The human AAA-ATPase Bcs1L translocates the fully assembled Rieske iron-sulfur protein (ISP) precursor across the mitochondrial inner membrane, enabling respiratory Complex III assembly. Bcs1L is a membrane-bound oligomer, with each subunit consisting of an N-terminal TM segment, a middle Bcs1-specific domain, and a C-terminal AAA domain that is highly distinct, forming a clade of its own in the broad AAA protein family. Here, we captured Bcs1L conformations by cryo-EM during active ATP hydrolysis in the presence or absence of ISP substrate. In contrast to the threading mechanism widely employed by AAA proteins in substrate translocation, subunits of Bcs1L alternate uniformly between ATP and ADP conformations without detectable intermediates that have different, co-existing nucleotide states, indicating that the subunits act in concert.

The quality of the density for the bound ADP was further enhanced in the map with applied C7 symmetry in the final refinement and reconstruction. To obtain the best resolution for the TM region of mBcs1L structures, we performed 3D reconstructions in C7 symmetry for the two ATP-bound maps (ATP state-1 and ATP state-2) and the ADP-bound map. These averaged maps reached higher resolution and allowed more structural features to be visualized in both ADP- and ATP-bound states. In the ADP state, the first 11 residues at the N-terminus (residues M1 to K11) form a 3-turn short helix, which lies parallel to the surface of MIM and is connected by a short loop to the 50 Å long, 9-turn TM helix (residues P14 to Y47) that spans the MIM (left). This N-terminal assembly consisting of the 3-turn short helix, the connecting loop, and the beginning (14PYF16) of the long TM helix makes contacts with their counterparts of neighboring subunits to form a seal on the IMS side of the membrane, hereafter referring to as IMS-Seal (left). The IMS-Seal in the ADP state features a narrow opening of ~9 Å in diameter, which is constructed by the side chains of Y15 pointing up and towards the center. In the apo/ADP states, the membrane basket in MIM is separated from the matrix cavity by the Matrix-seal that is parallel to the membrane plane. This seal is formed by the β-sheet I, protruding towards the center, with the central seal loops tightly packed together (bottom). In the apo/ADP conformation, both IMS-seal and Matrix-seal are closed.

>[7x]MPFSDFVLALKDNPYFGAGFGLVGVGTALAMARKGAQLGLVAFRRHYMITLEVPARDRSYAWLLSWLTRHSTRTQHLSVETSYLQHESGRISTKFEFIPSPGNHFIWYQGKWIRVERNRDMQMVDLQTGTPWESVTFTALGTDRKVFFNILEEARALALQQEEGKTVMYTAVGSEWRTFGYPRRRRPLDSVVLQQGLADRIVKDIREFIDNPKWYIDRGIPYRRGYLLYGPPGCGKSSFITALAGELEHSICLLSLTDSSLSDDRLNHLLSVAPQQSLVLLEDVDAAFLSRDLAVENPIKYQGLGRLTFSGLLNALDGVASTEARIVFMTTNYIDRLDPALIRPGRVDLKEYVGYCSHWQLTQMFQRFYPGQAPSLAENFAEHVLKATSEISPAQVQGYFMLYKNDPMGAVHNIESLRHHHHHH>[3x]VSKKPS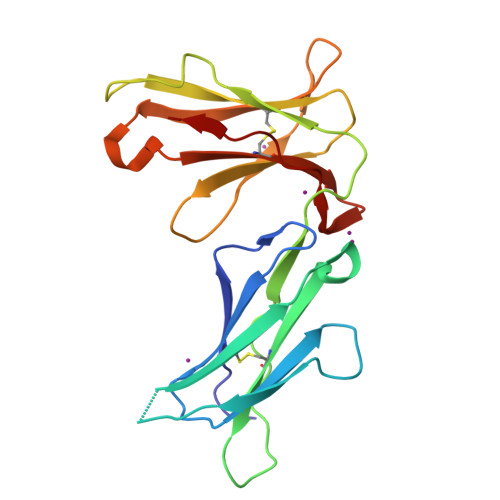LSVQPGPIVAPEETLTLQCGSDAGYNRFVLYKDGERDFLQLAGAQPQAGLSQANFTLGPVSRSYGGQYRCYGAHNLSSEWSAPSDPLDILIAGQFYDRVSLSVQPGPTVASGENVTLLCQSQGWMQTFLLTKEGAADDPWRLRSTYQSQKYQAEFPMGPVTSAHAGTYRCYGSQSSKPYLLTHPSDPLEL Aldo-keto reductases (AKRs) are a superfamily of oxidoreductases capable of reducing carbonyl to primary and secondary alcohols, found in all phyla. In this work, we identify the enzyme AKRtyl, which is responsible for tylosin reduction. Phylogenetic analysis indicates that AKRtyl is the founding member of subfamily D within family 12 in the AKR superfamily. Specifically, by combining steady-state and transient kinetics, X-ray crystallography and molecular dynamics simulation, we demonstrate that AKRtyl exhibits a positive synergy mediated by an unusual Monod-Wyman-Changeux (MWC) paradigm of allosteric regulation at low concentrations of the cofactor NADPH, but an inhibitory effect at high concentrations is observed.

Further, we added 1.2-times NADPH during AKRtyl crystallization, and the structure shows that the octamer exhibits an all-liganded active state (R4-N4R4-N4). Combined with other liganded states (R4-N2T4, R4-N4T4, R4-N1 R4-N1 as shown in Supplementary Fig. 13c–e), we find that the structure of the tetramers always exhibit symmetrical features. (2) The tetramer has structural symmetry in different ligand states (unliganded, partially liganded, fully liganded).

>[8x]MEYTQLGRIGLKVSRLVLGTMNFGPTTDEAESHAIMDAALDAGINFFDTANVYGWGENKGRTEEILGSWFAQGGDRRDKVVLATKVYGNMGLDGPAWPNHDKLSALNIRRSVDASLKRLGTDHIDLYQFHHVDRDTPWDEIWQAMDVLVRQGKILYVGSSNFAGWNIAQANETAARHGRLGLVSEQCLYNLCERRAEMEVVPAAREYGLGVIAWSPLHGGLLGGAIRKEQEGGNRRAASGRAADALKDPQQREQIQRYEDLLDKHGLEPGEVALAWLLTRPGVTGPIVGPRTADQLASAVRAAELTLTDEVLTALDEIFPGPGPSPEAFAW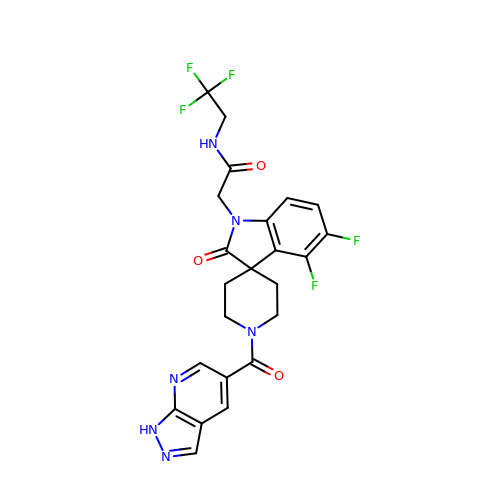2-[4,5-bis(fluoranyl)-2-oxidanylidene-1'-(1~{H}-pyrazolo[3,4-b]pyridin-5-ylcarbonyl)spiro[indole-3,4'-piperidine]-1-yl]-~{N}-[2,2,2-tris(fluoranyl)ethyl]ethanamide | C23 H19 F5 N6 O3 | IJPAFYMYOCLEBL-UHFFFAOYSA-N>MHHHHHHYFSINDSKILSLQNKKNTLMDTSGYNAEVRVEGNVQLNPIFPFDFKLGSSGDDRGKVIVTQNENIVYNAMYESFSISFWIRINKWVSNLPGYTIIDSVKNNSGWSIGIISNFLVFTLKQNENSEQDINFSYDISKNAAGYNKWFFVTITTNMMGNMMIYINGKLIDTIKVKELTGINFSKTITFQMNKIPNTGLITSDSDNINMWIRDFYIFAKELDDKDIN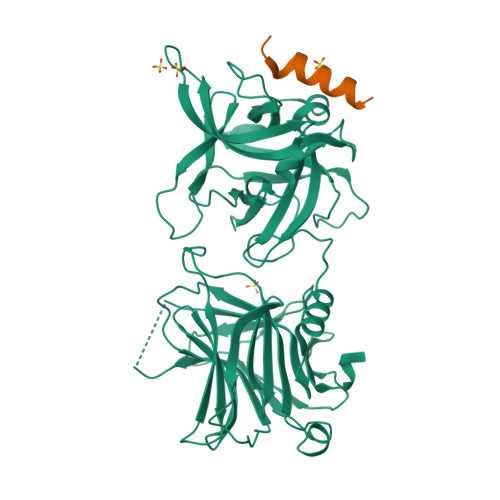ILFNSLQYTNVVKDYWGNDLRYDKEYYMINVNYMNRYMSKKGNGIVFNTRKNNNDFNEGYKIIIKRIRGNTNDTRVRGENVLYFNTTIDNKQYSLGMYKPSRNLGTDLVPLGALDQPMDEIRKYGSFIIQPCNTFDYYASQLFLSSNATTNRLGILSIGSYSFKLGDDYWFNHEYLIPVIKIEHYASLLESTSTHWVFVPAS[3x];>[3x]GESQEDMFAKLKDKFFNEINK> MVTIMHIEELLDIEDHGERDRQLRRYLAPYSAEIGVDGAEKMALVVLLNLTLKRDRVESLCDEGLARQLLSDEGHITNCLHTVRWLHTHNLKYPDARVSGERLIINAPPLIPGVISSAGLPMRMGWAHDSSDINLAKLFGTS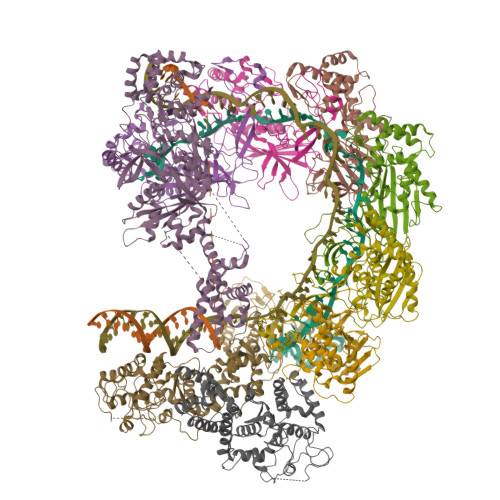FRYRDDSTNLALQLVARSKTWEQALIGLGLTQQQLDIWCQLLASNLENNTFPTVVSPFSKQVRFLYQGNYCVVTPVVSHALLAQLQNVVHEKKLQCTYIHHDHPASVGSLVGALGGKVAVLDYPPPVSPDKARSFSQARKHRLANGQSLFDRSVFNDHVFIDALKHVISRPGLTRKQQRQLRLSALRYLRRQLAIWLGPIIEWRDEIVSSGRGEPGNLPSGGLELELITQPKKMLPELMLQVAGRFHLELQNHSAGRRFAFHPALMAPIKSQILWLLRQLADDEEKDEPHPPTSCYYLHLSGLTVYDASALANPYLCGIPSLSALAGFCHDYERRLQSLIGQSVYFRGLAWYLGRYSLVTGKHLPEPSKSADPKSVSAIRRPGLLDGRYCDLGMDLIIEVHIPTGGSLPFTTCLDLLRVALPARFAGGCLHPPSLYEEYNWCTVYQDKSTLFTVLSRLPRYGCWIYPSDADLRSFEELSEALALDRRLRPVATGFVFLEEPVERAGSIEGQHVYAESAIGTALCINPVEMRLAGKKRFFGAGFWQLNDAKGAILMNGSANTG;>MELCTHLSYSRSLSPGKAVFFYKTAESDFVPLRIEVAKISGQKCGYTEGFDANLKPKNIERYELAYSNPQTIEACYVPPNVDELYCRFSLRVEANSMRPYVCSNPDVLRVMIGLAQAYQRLGGYNELARRYSANVLRGIWLWRNQYTQGTKIEIKTSLGSTYHIPDARRLSWSGDWPELEQKQLEQLTSEMAKALSQPDIFWFADVTASLKTGFCQEIFPSQKFTERPDDHSVASRQLATVECSDGQLAACINPQKIGAALQKIDDWWANDADLPLRVHEYGANHEALTALRHPATGQDFYHLLTKAEQFVTVLESSEGGGVELPGEVHYLMAVLVKGGLFQKGKGR[6x];> MTENRYFFAIRYLSDDVDCGLLAGRCISILHGFRQAHPGIQIGVAFPEWSDRDLGRSIAFVSTNKSLLERFRERSYFQVMQADNFFALSLVLEVPDTCQNVRFIRNQNLAKLFVGERRRRLARAKRRAKARGEAFQPHMPDETKVVGVFHSVFMQSASSGQSYILHIQKHRYERSEDSGYSSYGLASNDLYTGYVPDLGAIFSTLF;>[2x]MHLLVRPEPFADEALESYFLRLSQENGFERYRIFSGSVQDWLHTTDHAAAGAFPLELSRLNIFHASRSSGLRVRALQLVDRLTDGAPFRLLQLALCHSAISFGNHYKAVHRSGVDIPLSFIRVHQIPCCPDCLRESAYVRQCWHFKPYVGCHRHGGRLIYSCPACGESLNYLASESINHCQCGFDLRTASTVPAQPDEIQLSALAYGCSFESSNPLLAIGSLSARFGALYWYQQRYLSDHEAVRDDRALTKAIGHFTAWPDAFWRELQQMVDDALVRQTKPLNHTDFVDVFGSVVADCRQIPMRNTGQNFILKNLIGFLTDLVARHPQCRVANVGDLLLSAVDAATLLSTSVEQVRRLHHEGFLPLSIRPASRNTVSPHRAVFHLRHVVELRQARMQSHHDHSSTYLPAW> 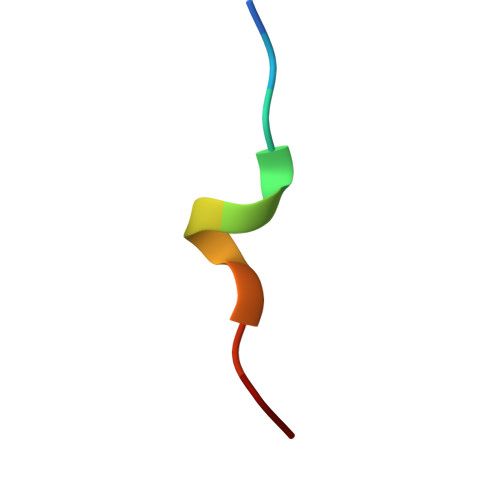GSDITRFLVKK We present in this paper the structure of two additional archaeal T4P, one from Pyrobaculum arsenaticum, a neutrophilic hyperthermophile (optimal growth at 90 °C, pH 7) and the other from Saccharolobus solfataricus, an acidophilic hyperthermophile (optimal growth at 75–80 °C, pH 2-3). Although the full spectrum of functions played by archaeal T4P is yet to be uncovered, they are known to mediate adhesion to various biotic and abiotic surfaces, and play an important role in DNA exchange, intercellular communication and biofilm formation. Finally, we show that Pyrobaculum and the Saccharolobus T4P are at the forefront of virus-host interaction and are recognized by two different viruses, likely serving as primary receptors during virus infection. We show that whereas the N-terminal domain is conserved in all bacterial and archaeal T4P-like filaments, the C-terminal domain of bacterial T4P is unrelated to the immunoglobulin (Ig)-like domain shared by archaeal T4P and archaeal flagella.

The S. solfataricus pilus was very similar to that of S. islandicus, albeit at considerably higher resolution (3.4 versus 4.1 Å), which was not surprising given the ~81% sequence identity between the two. While multiple helical symmetries appeared to be possible based upon analysis of power spectra from these filaments, in each case only one helical symmetry led to a reconstruction with clearly interpretable secondary structure. This was a rise of ~5.3 Å and a rotation of ~101.7° for the P. arsenaticum filaments and a rise of ~5.0 Å and a rotation of ~104.6° for the S. solfataricus filaments. The small difference in helical twist between the two resulted in 7-start long-pitch helices that were left-handed for P. arsenaticum and right-handed for S. solfataricus. However, in P. arsenaticum pilus, there are slightly more than 3.5 subunits per turn, so there are 7.1 subunits in two turns, while in S. solfataricus there are slightly less than 3.5 subunits per turn, yielding 6.9 subunits in two turns. In the S. solfataricus pilin, similar to S. islandicus, only about 1.5% of the residues are charged. In S. solfataricus and S. islandicus, ~37% of the residues in the globular domain are either serine or threonine, potential sites for O-linked glycosylation. In S. solfataricus, we see clear extra density consistent with glycosylation on seven residues, all serines or threonines. There was no apparent glycosylation of this virus, and the small extra density not explained by the atomic model involves a few disordered C-terminal residues of the capsid protein that were not part of the atomic model. It can be seen that, as expected, the S. solfataricus filament has a significantly greater amount of peripheral density due to glycosylation than the P. arsenaticum filament. Whereas binding of SSRV1 to S. solfataricus pili is likely to be mediated through carbohydrate moieties, direct interaction with the pilin subunits might play an important role in the case of PFV2.

>LSGAVTALILVIASVIIALVVVGFAFGLFGAFTGQGTVAQVGTATLSASTLTLTVTLKNTGASTQVTGVLINGNSGSVSGMTTISAGVNTYTITISIGSISTTLRGLVGSTISLTLILSNGETVTVSAIVTS[33x]> ASGLVPRGSHMMEILRGSPALSAFRINKLLARFQAANLQVHNIYAEYVHFADLNAPLNDSEQAQLTRLLQYGPALSSHTPAGKLLLVTPRPGTISPWSSKATDIAHNCGLQQVDRLERGVAYYIEASTLTAEQWRQVAAELHDRMMETVFSSLTDAEKLFIHHQPAPVSSVDLLGEGRQALIDANLRLGLALAEDEIDYLQEAFTKLGRNPNDIELYMFAQANSEHCRHKIFNADWIIDGKPQPKSLFKMIKNTFETTPDYVLSAYKDNAAVMEGSAVGRYFADHNTGRYDFHQEPAHILMKVETHNHPTAISPWPGAATGSGGEIRDEGATGRGAKPKAGLVGFSVSNLRIPGFEQPWEEDFGKPERIVTALDIMTEGPLGGAAFNNEFGRPALTGYFRTYEEKVNSHNGEELRGYHKPIMLAGGIGNIRADHVQKGEIVVGAKLIVLGGPAMNIGLGGGAASSMASGQSDADLDFASVQRDNPEMERRCQEVIDRCWQLGDANPILFIHDVGAGGLSNAMPELVSDGGRGGKFELRDILSDEPGMSPLEIWCNESQERYVLAVAADQLPLFDELCKRERAPYAVIGDATEEQHLSLHDNHFDNQPIDLPLDVLLGKTPKMTRDVQTLKAKGDALNRADITIADAVKRVLHLPTVAEKTFLVTIGDRTVTGMVARDQMVGPWQVPVADCAVTTASLDSYYGEAMSIGERAPVALLDFAASARLAVGEALTNIAATQIGDIKRIKLSANWMAAAGHPGEDAGLYDAVKAVGEELCPQLGLTIPVGKDSMSMKTRWQEGNEQREMTSPLSLVISAFARVEDVRHTLTPQLSTEDNALLLIDLGKGHNALGATALAQVYRQLGDKPADVRDVAQLKGFYDAMQALVAARKLLAWHDRSDGGLLVTLAEMAFAGHCGVQVDIAALGDDHLAALFNEELGGVIQVRAEDRDAVEALLAQYGLADCVHYLGQALAGDRFVITANDQTVFSESRTTLRVWWAETTWQMQRLRDNPQCADQEHEAKANDTDPGLNVKLSFDINEDIAAPYIATGARPKVAVLREQGVNSHVEMAAAFHRAGFDAIDVHMSDLLGGRIGLGNFHALVACGGFSYGDVLGAGEGWAKSILFNHRVRDEFETFFHRPQTLALGVCNGCQMMSNLRELIPGSELWPRFVRNHSDRFEARFSLVEVTQSPSLLLQGMVGSQMPIAVSHGEGRVEVRDDAHLAALESKGLVALRY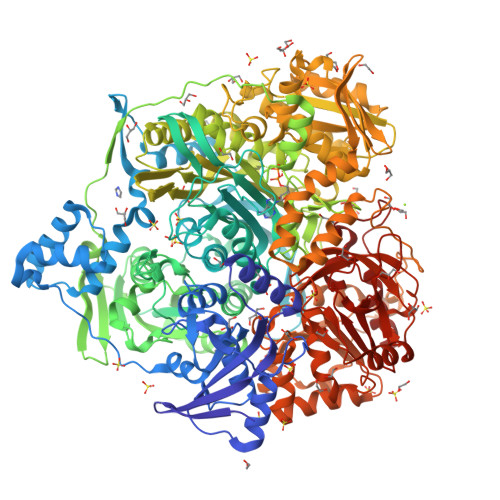VDNFGKVTETYPANPNGSPNGITAVTTENGRVTIMMPHPEAVFRTVANSWHPENWGEDSPWMRIFRNARKQLG> MYIGKPIKRIEDLRLITGKGAYVDDIELPGTLFVAFVRSKYPHARIKVKKEEGIFTGEDINPGKDFPIATKETTYVGQPIAIVIAKDRYEAYDLIESVEVEYEELDYVLDPEKALEDKVKVHSGLSSNIYYHERWKGGDVEKAFKEADLTISDTLINQRVIASPLETRGALAYFDGNKLTFYSSTQSAHYLRRNLVDFLGFENIRVIQPDVGGAFGSKIIAHPEEYALAKLALMLRKPLKWVPTRTEEFISAGHGRDKKLKFEVAVKKDGTILGIRGTLIANLGAPYPDANDDESGNVKSTVRMLPGIYKIIGADIDAYAVHTNITPTQSYRGAGRPEGIYFIERIVNIVADELGIDQYEIRLKNAIDTLPYTNIFGVTYDSGNVKKLLEIGKKYYDELKKEDGCVGVSSYIEITAFGPWEVARISVKYDGKITLVTGTGPHGQGDATAFAQIAADVLELPIEKIEVRWGDTEIIEDGIGTWGSRT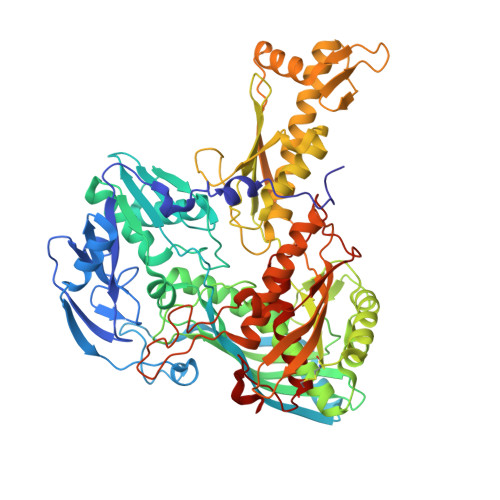VTIGGSAVLLASQKLKDKLIEIGAKILNADKEEVEYKEGNVTHKKNGNKVTFNEIVKNAFKMGESLDTTAIYNVKQPPTTPYGVHLALVKVDGTGKVFVKKYVAVDDVGTVINPLLAEGQAIGGIVQGMAQALLEGAFFDENGQLLTTNFQDYPIPTAVEIPEKIDWYYEILGKSPHPTGSKGIGEAGAIAATPTIINAVEQCIKKRITKMPVKFEELVS> IVGGQDATRGMFPYQLSLQHMGAGWYHTCGAILLAANKALTAAHCTEGREGFRVLAGAHVLPANDQEQESDVASVTEHPEFDRFGPGIPNDVATMALATAINAAGNVGYATLAAANAPDYAGDQARLSGWGKLHGADDGIADTLQYVVTTVRSTADCNARMPEHIQNVMDQHICVHSDTGTTGSCQGDSGGPMTHGASGSGNVIGVTSWGIGNPVESCLPDFPSVYARVSYFRAWIDAN

Here, we introduce a small facultative plasminogen-independent thrombolytic enzyme, snFPITE, isolated from Sipunculus nudus. Compared to traditional thrombolytic agents, snFPITE does not require plasminogen for thrombolysis, although its presence enhances lytic activity. Native/SDS-PAGE, high-resolution mass spectrometry (HRMS), and ultrahigh-performance liquid chromatography (UHPLC) unveiled that snFPITE was a small monomer protein with a molecular weight of 24.925 kD. Mechanistically, snFPITE activates plasminogen and degrades fibrin(ogen) in a multisite cleavage manner. snFPITE is inhibited by plasminogen activator inhibitor 1 and α2-antiplasmin via a competitive inhibition.

Prior to crystallization, the protein samples were treated with the serine protease inhibitor phenylmethylsulphonylfluoride (PMSF). This treatment facilitated the clear observation of electron densities corresponding to the PMSF molecule covalently bonded to Ser189 of snFPITE-n1, snFPITE-n2-A, and snFPITE-n2-B within the PMSF-snFPITE-n1/n2 cocrystal structures. Based on protein sequence alignment, the closest homolog of snFPITE-n1 was found to be the fibrinolytic enzyme from Enchytraeus japonensis (44% identity). High-resolution crystal structures of both snFPITE-n1 and snFPITE-n2 reconfirmed that their catalytic triads consisted of His44, Asp91, and Ser189, and the weak substrate specificity might be caused by Gly183 and Ile88 residues in the binding pockets S1 and S2, or the four additional residues (Cys, Leu, Pro, and Asp) inserted into the S1 pocket of snFPITEs. Notably, both Asp91 and Ser189 established hydrogen bonds with His44, a feature that is essential for facilitating the catalytic interaction. Furthermore, the model of snFPITE-n1 complexed with a canonical human plasminogen peptide displayed that a steric clash between the peptide and snFPITE-n1 was absent, suggesting that this peptide could be an appropriate substrate for snFPITE-n1. This peptide was bound to snFPITE-n1 with the Arg580 residue inserted into the negatively charged pocket, as in tPA. Meanwhile, six snFPITE-n1 models with six 7-mer peptide substrates from α, β, and γ chains of fibrinogen revealed the absence of steric clash between snFPITE-n1 and these peptide substrates, suggesting that snFPITE-n1 could accommodate substrates from the fibrinogen chains. In all these models, the Lys or Arg residue was buried in the negatively charged pocket. Meanwhile, the pockets of snFPITE-n1, which were less charged than those of tPA and plasmin, were compatible with the broader substrate selectivity of this enzyme.> UUUUUCAGUUAGAGCGUCGUGUCUCUUGUACGUCUCGGUCACAAUACACGGUUUCGUCCGGUGCGUGGCAAUUCGGGGCACAUCAUGUCUUUCGUGGCUGGUGUGACCGCGCAAGGUGCGCGCGGUACGUAUCGAGCAGCGCUCAACUCUGAAAAA

SL5 is the largest and most complex structural element in the 5′-proximal regions of βCoV RNA genomes. We further determined the 3D structures of the SL5 elements from these representatives using single-particle cryo-EM, which revealed remarkable structural similarity despite the low sequence conservation and variable lengths. All four structures exhibited a T-like shape, with the topology of the junctions featuring the SL5 basal stem positioned almost at right angles to the coaxial stack of SL5a/SL5b stems. Overall, the SL5 elements exhibited remarkable global structure conservation, despite the divergence at the level of individual nucleotide residues and their base pairs.

Cryo-EM single particle analyses generated high-quality 2D class averages and maps at 7.1, 6.5, 5.9, 6.6 Å overall resolutions for OC43-CoV, SARS-CoV-2, MERS-CoV, and RoBat-CoV, respectively. Our results provided detailed insights into the SL5 3D structure, revealing a 4WJ architecture in OC43-CoV, SARS-CoV-2, and MERS-CoV, and a 3WJ in RoBat-CoV. The SL5 4WJ in OC43-CoV, SARS-CoV-2, MERS-CoV was formed by four canonical base pairs, coming from the four stems, while in RoBat-CoV the SL5 3WJ was formed by two canonical pairs and one G–U wobble pair. In SARS-CoV-2 and MERS-CoV RNAs, the base pairs at the junction motif were the same. The junctions of SARS-CoV-2 and MERS-CoV were most similar to each other, with an RMSD of 2.36 Å. Coronaviruses possess one (like MERS-CoV) or two (as in SARS-CoV-2 and RoBat-CoV) copies of this motif, situated within structural elements. In MERS-CoV, the GCGUG motif is located in the SL5a, near the loop. Distinct SL5 shapes were identified, such as the Y-shape in OC43-CoV, the more compact blob-like shape in MERS-CoV and SARS-CoV-2, and the rod-like shape in RoBat-CoV, in strong agreement with the cryo-EM maps of SL5. MERS-CoV had the lowest Tm, while RoBat-CoV had the highest, likely due to its fewer single-stranded regions.> MDHHHHHHHHTSETGYVQGTEKQLSCCLDLMRRLPPSQIEDNLAGLLDLVPDLTEDLLSSIDQPLKVAYDAVSKKDYLLCDYNRDADSYRSPWSNKYDPPLSGACYPSSKLRDIEVQANEIFEIYLNLYFEGGVSSVYCWDLDDNFAAVVLMKKTQDQSKKGQPMRGTWDSIHVVEVKLGKKDKAVYKLTSTVMLSIETDNDNT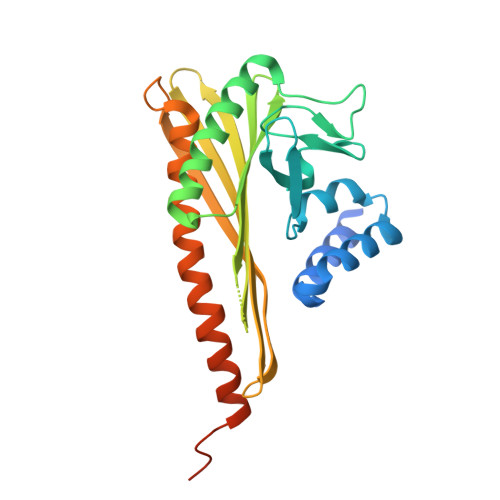GKVNLAGSLTRQDEKEYTFNEVDTHCVNIGKMVEDMESKLRQTLETIYFGKTKEVVNTLRNATGNSELEKRKNLSNQIGSAIGNRG> IEIPKEVTEEGKNVYKKYCAPCHGEEGGGDGLLSRSMLPKPRNFTLGAYKFRTTPSGSLPTDEDIYRTISYGVPNSTMIPWDILTEEQRASVVPVLKS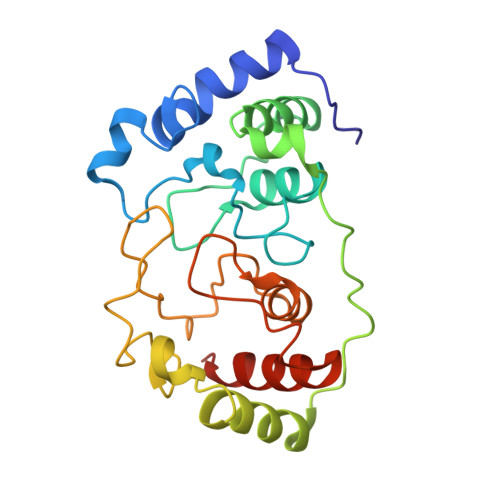FSEAFEYREPEPSVDVGLPLRPTERTILAGKKIYEEKLECWKCHGVEGRGDGPSASEQEDDFGFPIKPFDFTTGKFKGGNSPTDVYLRFTTGLNGTPMPSFAKELSDDERWYLTHYVMSLVQPEKCRK> EDPEGSRITYVKGDLFACPKTDSLAHCISEDCRMGAG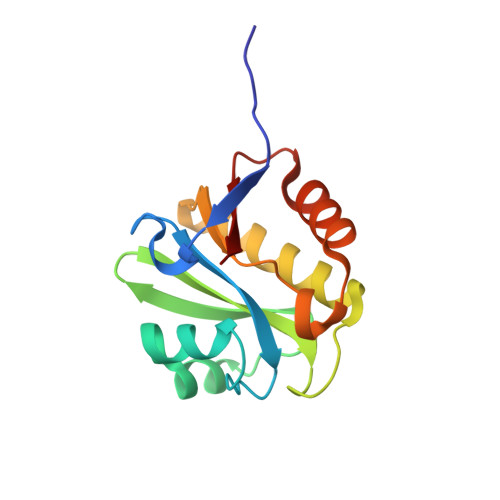IAVLFKKKFGGVQELLNQQKKSGEVAVLKRDGRYIYYLITKKRASHKPTYENLQKSLEAMKSHCLKNGVTDLSMPRIGCGLDRLQWENVSAMIEEVFEATDIKITVYTL The upstream region of a riboswitch is the aptamer domain, a highly structured sequence generally found in bacterial mRNA leader sequences, that specifically binds a small organic metabolite or cation. The occupancy status of the aptamer domain is communicated to a downstream expression platform that directs expression machinery. Structural and biochemical analyses of the aptamer domain of several representative members, including the guanine riboswitch that regulates the xpt-pbuX transcriptional unit in Bacillus subtilis, has revealed a binding pocket that is almost completely solvent inaccessible and forms hydrogen bonds with all of the ligand’s polar groups. The B. subtilis xpt-pbuX guanine riboswitch is an “OFF” switch in which ligand binding promotes the formation of an intrinsic terminator, causing RNA polymerase to disengage from mRNA synthesis.

Discrimination between guanine and adenine is conferred by the pyrimidine residue at position 74 (nucleotide numbering used throughout this work is that of the B. subtilis xpt guanine riboswitch) via the Watson–Crick base pairing with the ligand. In the guanine-bound form, both hydrogens of the N2-amino group engage in hydrogen bonding interactions with carbonyl oxygens of U51 and C74; modifications at the C2 position would require the disruption of interactions with one of the pyrimidine residues. The crystal structures of the guanine and adenine riboswitches reveal that the ligand’s C8 is less than 3.5 Å distance from three nucleotides (A21, U22 and A47), suggesting that there is insufficient room in the purine ligand bound binding pocket to accommodate any functional group at this site. By ITC, guanine binds GR(A19C-U77G) RNA with a KD of 0.85 ± 0.31 nM, a ~2.5-fold higher affinity than the wild-type GR. The comparison of the transcription of the xpt gene in the absence and presence of 20 µM guanine reveals a modest ability to repress read-through transcription (48% and 77% terminated product, respectively). The superposition of nucleotides around the binding pocket (nts 20–24, 46–53 and 73–76) and the ligand reveals that 8-aminoguanine and adjacent residue C74 are displaced by ~0.3 Å, only slightly greater than the maximum likelihood coordinate errors in each structure (0.16 and 0.24 Å). The crystal structure of GR bound to guanine and N2-acetylguanine superimpose very well (r.m.s.d. = 0.33 Å), indicating that this analog does not disrupt the global architecture. Instead, these data argue that there may be multiple pathways to form the crystallographically observed ligand-GR complex. In the case of guanine and adenine binding, the above pathway that is supported by a wealth of biochemical and structural data is likely highly populated.

> GGACAUAUAAUCGCGUGGAUAUGGCACGCAAGUUUCUACCGGGCACCGUAAAUGUCCGACUAUGUCC GBS strains express either one of two SRR proteins, Srr1 or Srr2. We now report that both Srr1 and Srr2 bind to a specific tandem repeat region of fibrinogen Aα chain. As was previously predicted from sequence and functional analyses, Srr1-BR and Srr2-BR each adopt an overall fold that resembles the binding regions of “microbial surface components recognizing adhesive matrix molecules” (MSCRAMMs), including the well characterized ClfA, ClfB, SdrG, and the likely MSCRAMM UafA. Like other MSCRAMMs, Srr1-BR and Srr2-BR contain two domains, termed N2 and N3, with each adopting the DE variation of the Ig fold.

To assess whether Srr1 and Srr2 could support a DLL mechanism of ligand binding, we determined the crystal structures of S. agalactiae Srr1-BR and Srr2-BR at resolutions of 1.65 and 3.65 Å, respectively. However, Srr1-BR and Srr2-BR are more similar to each other than they are to these structurally characterized MSCRAMMs, with a root mean square deviation of 1.6 Å between Srr1-BR and Srr2-BR and root mean square deviations between 2.1 and 2.5 Å when either Srr1 or Srr2 is placed in a pairwise structural alignment with ClfA, ClfB, SdrG, or UafA. Notably, a bulky amino acid of the N3 domain (Tyr-623 of Srr1 and His-528 of Srr2) significantly constricts the center of each trench. In addition, we have recently shown that Srr1 binds to human fibrinogen via its interaction with the Aα chain of the protein. Sequence comparisons and deletion mutagenesis studies suggest that the interaction between Srr1 and fibrinogen could employ the “dock, lock, and latch” (DLL) mechanism described for several other fibrinogen-binding adhesins, such as ClfB of S. aureus and SdrG of Staphylococcus epidermidis. Deletion of the latch region of Srr1 is associated with reduced GBS binding in vitro to fibrinogen and hBMEC and resulted in attenuated virulence in a mouse model of bacteremia and meningitis. Alignment of the Srr1- and Srr2-predicted latching clefts with those of other DLL adhesins showed that Srr1 has closer homology to these other DLL proteins, as compared with Srr2. To address this possibility, we constructed variants of the Srr1 and Srr2 BRs, in which residues in both the latch and latching cleft regions were replaced with a cysteine, such that a disulfide bond would be formed, thus fixing the spatial position of the latch. Under reducing conditions (1 mm DTT), the mutant proteins had mobilities identical to their WT counterparts As compared with the WT Srr1-BR and the Srr2 BR, both cross-linked proteins showed enhanced binding to fibrinogen. These data indicate that the affinities of Srr1 and Srr2 for fibrinogen are enhanced by a pre-closed latch, consistent with the location of the latch influencing binding affinity.

> MEVSDTEMLGKDVSSELQKVNIALKDNTLSEPGTVKLDSSENLVLNFAFSIASVNEGDVFTVKLSDNLDTQGIGTILKVQDIMDETGQLLATGSYSPLTHNITYTWTRYASTLNNIKARVNMPVWPDQRIISKTTSDKQCFTATLNNQVASIEERVQYNSPSVTEHTNVKTNVRSRIMKLDDERQTETYITQINPEGKEMYFASGLGNLYTIIGSDGTSGSPVNLLNAEVKILKTNSKNLTDSMDQNYDSPEFEDVTSQYSYTNDGSKITIDWKTNSISSTTSYVVLVKIPKQSGVLYSTVSDINQTYGSKYSYGHTNISGDSDANAEIKLLLEHHHHHH>MGSDKIHHHHHHENLYFQGMYPDLVHLGGADKYFEEILEIVNKIKLFGDFSNEEVRYLCSYMQCYAAPRDCQLLTEGDPGDYLLL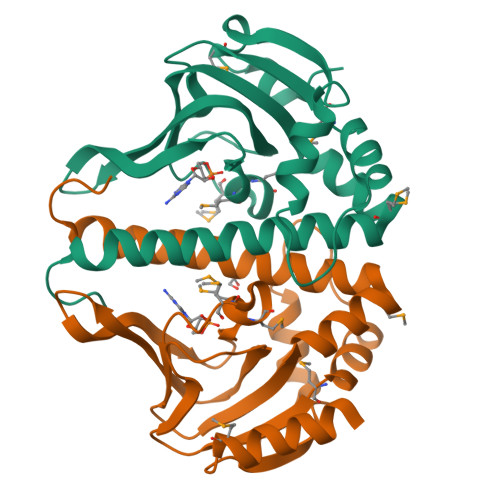ILTGEVNVIKDIPNKGIQTIAKVGAGAIIGEMSMIDGMPRSASCVASLPTDFAVLSRDALYQLLANMPKLGNKVLIRLLQLLTARFRESYDRILPKTLGELI[2x]> SNAKLLAITSCPNGIAHTYMAAENLQKAADRLGVSIKVETQGGIGVENKLTEEEIREADAI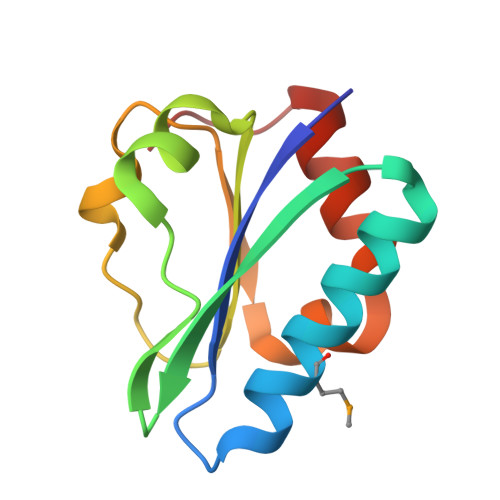IIAADRSVNKDRFIGKKLLSVGVQDGIRKPEELIQKALNGDIPVY1-{4-[4-(2-ethoxyphenyl)piperazin-1-yl]-1,3,5-triazin-2-yl}piperidine-4-carboxylic acid | C21 H28 N6 O3 | 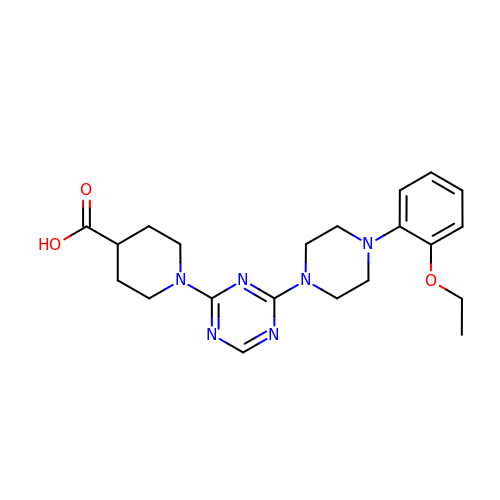MFDIQEKYAZCUMU-UHFFFAOYSA-N>[2x]MGRDLRDNETWWY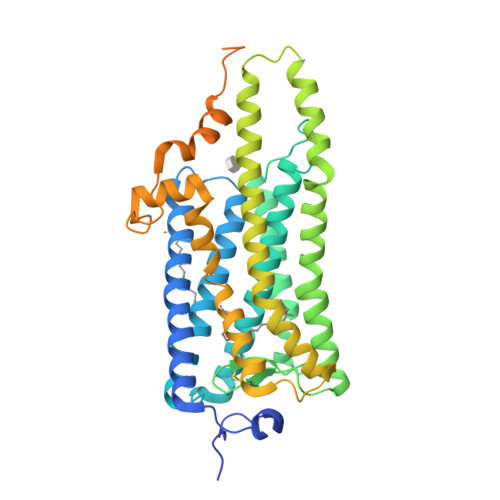NPSIVVHPHWREFDQVPDAVYYSLGIFIGICGIIGCGGNGIVIYLFTKTKSLQTPANMFIINLAFSDFTFSLVNGFPLMTISCFLKKWIFGFAACKVYGFIGGIFGFMSIMTMAMISIDRYNVIGRPMAASKKMSHRRAFIMIIFVWLWSVLWAIGPIFGWGAYTLEGVLCNCSFDYISRDSTTRSNILCMFILGFFGPILIIFFCYFNIVMSVSNHEKEMAAMAKRLNAKELRKAQAGANAEMRLAKISIVIVSQFLLSWSPYAVVALLAQFGPLEWVTPYAAQLPVMFAKASAIHNPMIYSVSHPKFREAISQTFPWVLTCCQFDDKETEDDKDAETEIPAGESSDAAPSADAAQMKEMMAMMQKMQQQQAAYPPQGYAPPPQGYPPQGYPPQGYPPQGYPPQGYPPPPQGAPPQGAPPAAPPQGVDNQAYQA>HHHHHHMTDKTLQQIDKLICSWLKQIDNVIPQLIMEMTTETKRHRFDLVTNVDKQIQQQFQQFLATYFPEHQLLAEEKSNAMITNEINHLWIMDPIDGTANLVKQQEDYCIILAYFYEGKPMLSYVYDYPHKKLYKAIRGEGAFCNGIKMEEPPSLKLEDAIISFNAQVMNLDTVQDLFDASFSYRLVGACGLDSMRVAKGQFGAHINTNPKPWDIAAQFLFAELLNLKMTTLDGKAIDHLKGAPFIISNKACHETVLKIL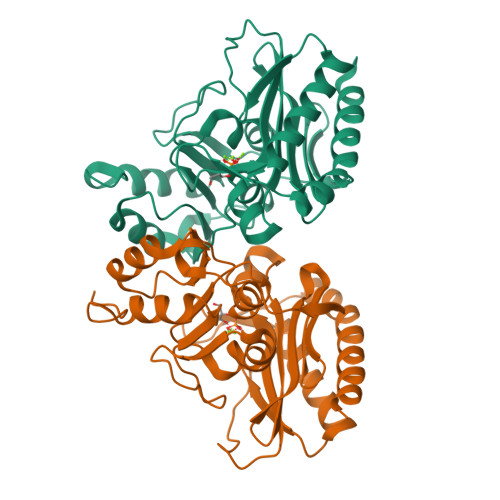NANGGYQKYR[2x]>[5x]HMMPSEDYAIWYARATIAALQAAEYRLAMPSASYTAWFTDAVS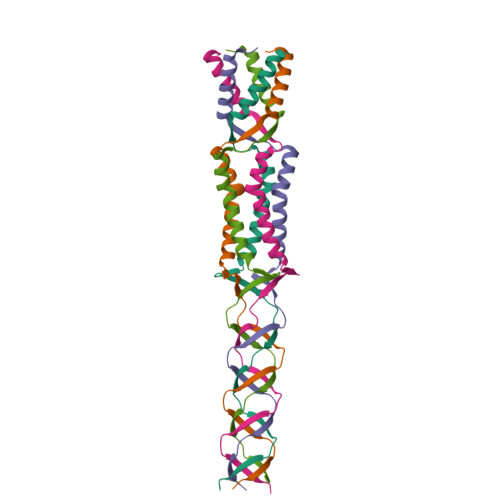DKLDKISESLNTLVECVIDKRLAVSVPEPLPVRVENKVQVEVEDEVRVRVENKVDVEVKN> MIQQTGYSKKVMEHFMNPRNVGVIDDPDGYGKVGNPVCGDLMEIFIKVGDEKI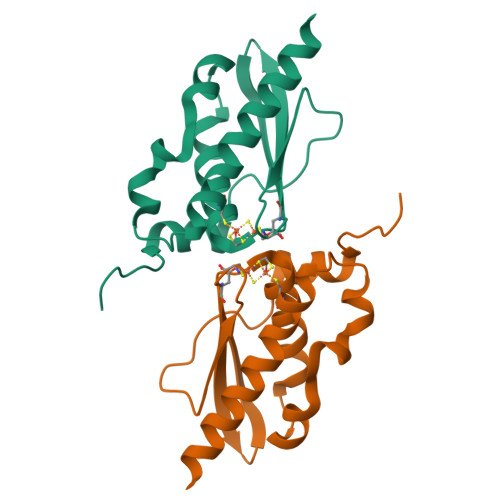EDIKFRTFGCGAAIATSSMITEMARGKSLEEAMRITRNDVADALDGLPPQKMACSNLAADALHAAINDYLSKKQKHLEHHHHHH>[2x]GEIPTIGQQMETGDQRFGDLVFRQLAPNVWQHTSYLDMPGFGAVASNGLIVRDGGRVLVVDTAWTDDQTAQILNWIKQEINLPV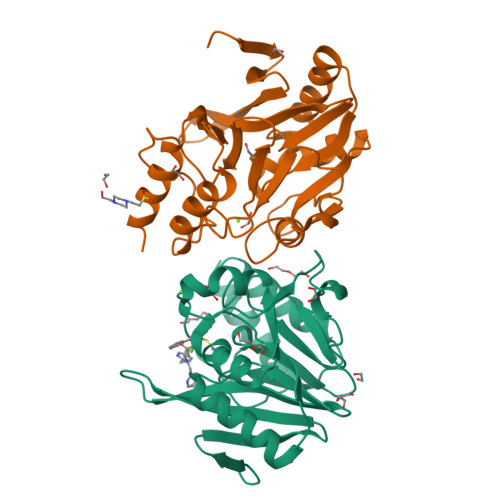ALAVVTHAHQDKMGGMDALHAAGIATYANALSNQLAPQEGMVAAQHSLTFAANGWVEPATAPNFGPLKVFYPGPGHTSDNITVGIDGTDIAFGGCLIKDSKAKSLGNLGDADTEHYAASARAFGAAFPKASMIVMSHSAPDSRAAITHTARMADKLR>PMFIVNTNVPRASVPDGFLSELTQQLAQATGKPPQYIAVHVVPDQLMAFGGSSEPCALCSLHSIGKIG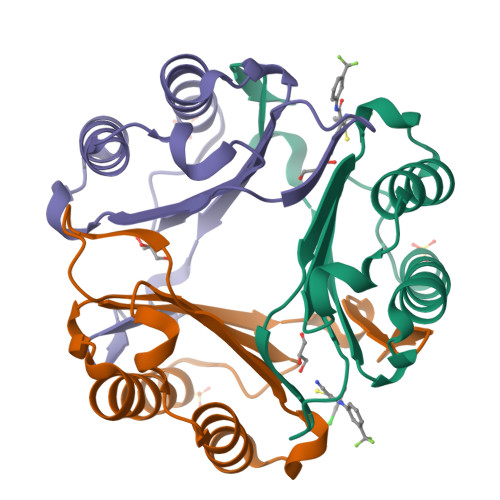GAQNRSYSKLLCGLLAERLRISPDRVYINYYDMNAANVGWNNSTFA[3x]> AMLPISMSDEGDSFLVKDSLGENKIPKNPSKVVILDLGILDTFDALKLNDKVVGVPAKNLPKYLQQFKNKPSVGGVQQVDFEAINALKPDLIIISGRQSKFYDKLKEIAPTLFVGLDNANFLSSFENNVLSVAKLYGLEKEALEKISDIKNEIEKAKSIVDEDKKALIILTNSNKISAFGPQSRFGIIHDVLGINAVDENIKVGTHGKSINSEFILEKNPDYIFVVDRNVILGNKERAQGILDNALVAKTKAAQNKKIIYLDPEYW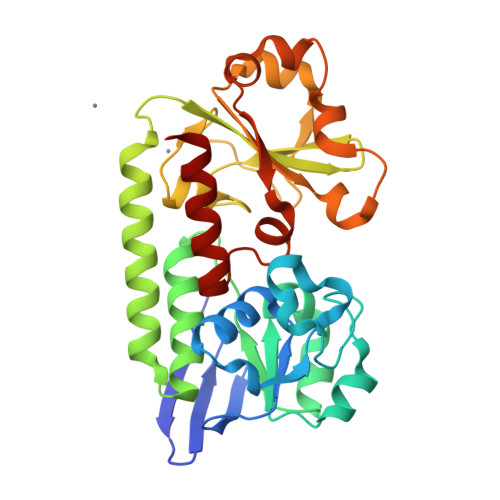FLASGNGLESLKTMILEIKNAVK>MAHHHHHHMRRVVITGLGLVSPLASGVEETWKRLLAGESGARRVTEFEVDDLACQIACRIPVGDGTNGTFNPDLHMDPKEQRKVDPFIVYAVGAADQALDDAGWHPENDEDQVRTGVLIGSGIGGIEGIVEAGYTLRDKGPRRISPFFIPGRLINLASGHVSIKHKLRGPNHSVVTACATGTHAIGDAARLIAFGDADVMVAGGTESPVSRISLAGFAACKALSTERNDDPTAASRPYDEDRDGFVMGEGAGIVVLEELEHALARGAKIYAEVIGYGMSGDAFHITAPTESGEG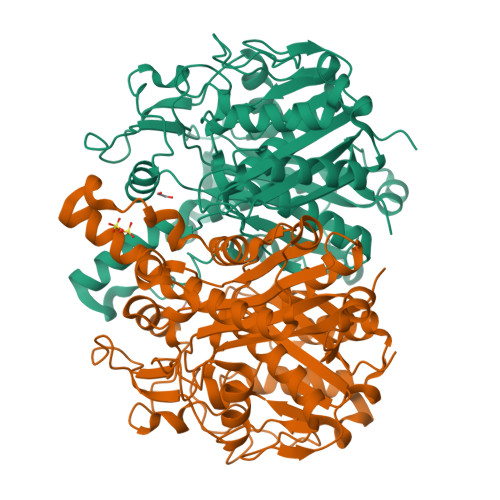AQRCMVAALKRAGIVPDEIDYINAHGTSTMADTIELGAVERVVGEAAAKISMSSTKSSIGHLLGAAGAAEAVFSTLAIRDNIAPATLNLDNPAAQTRIDLVPHKPRERKIDVALSNSFGFGGTNASLVLRRYTA[3x]>MAHHHHHHVGTFENITAAPADPILGLADLFRADERPGKINLGIGVYFDETGKIPVLTSVKKAEQYLLENETTKYYLGIDGIPEFGRCTQELLFGKGSALINDKRARTAQTPGGTGALRVAADFLAKNTSVKRVWVSNPSWPNHKSVFNSAGLEVREYAYYDAENHTLDFDALINSLNEAQAGDVVLFHGCCHNPTGIDPTLEQWQTLAQLSVEKGWLPLFDFAYQGFARGLEEDAEGLRAFAAMHKELIVASSYSKNFGLYNERVGACTLVAADSETVDRAFSQMKAAIRANYSNPPAHGASVVATILSNDALRAIWEQELTDMRQRIQRMRQLFVNTLQEKGANRDFSFIIKQNGMFSFSGLTKEQVLRLREEFGVYAVASGRVNV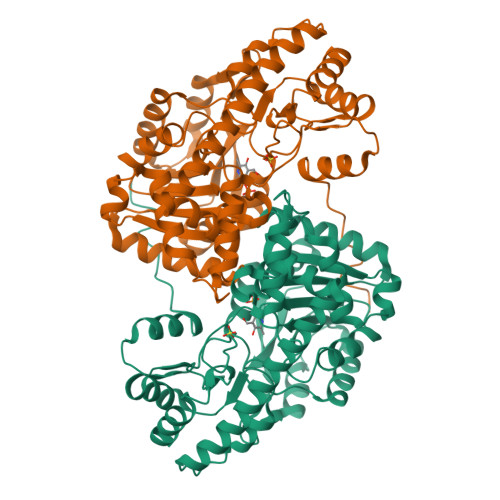AGMTPDNMAPLCEAIVAVL[2x]> MKPRACVVVYPGSNCDRDAYHALEINGFEPSYVGLDDKLDDYELIILPGGFSYGDYLRPGAVAAREKIAFEIAKAAERGKLIMGICNGFQILIEMGLLKGALLQNSSGKFICKWVDLIVENNDTPFTNAFEKGEKIRIPIAHGFGRYVKIDDVNVVLRYVKDVNGSDERIAGVLNESGNVFGLMPHPERAVEELIGGEDGKKVFQSIL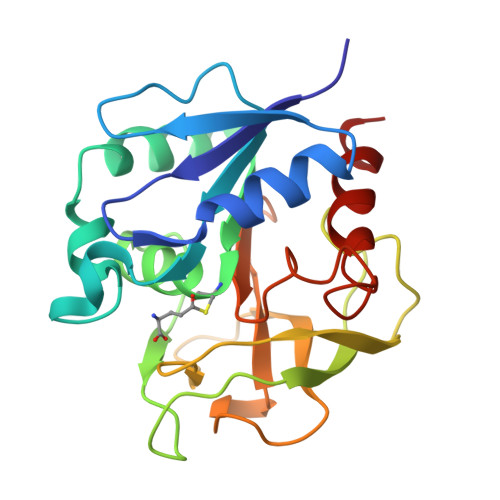NYLKR> PLPTGYFGIPLGLAALSLAWFHLENLFPAARMVSDVLGIVASAVWILFILMYAYKLRYYFEEVRA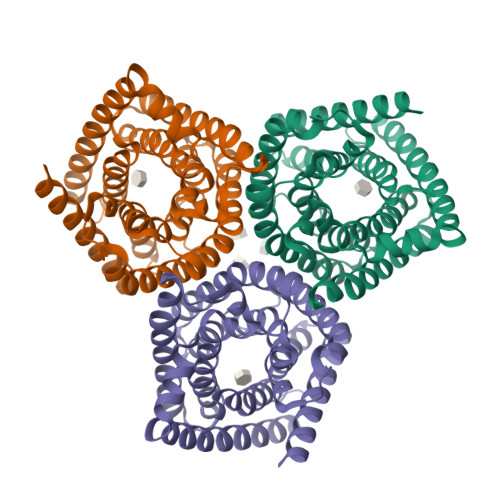EYHSPVRFSFIALIPITTMLVGDILYRWNPLIAEVLIWIGTIGQLLFSTLRVSELWQGGVFEQKSTHPSFYLPAVAANFTSASSLALLGYHDLGYLFFGAGMIAWIIFEPVLLQHLRISSLEPQFRATMGIVLAPAFVCVSAYLSINHGEVDTLAKILWGYGFLQLFFLLRLFPWIVEKGLNIGLWAFSFGLASMANSATAFYHGNVLQGVSIFAFVFSNVMIGLLVLMTIYKL>MRSRRVDVMDVMNRLILAMDLMNRDDALRVTGEVREYIDTVKIGYPLVLSEGMDIIAEFRKRFGCRIIADFKVADIPETNEKICRATFKAGADAITVHGFPGADSVRACLNVAEEMGREVFLLTEMSHPGAEMFIQGAADEIARMGVDLGVKNYVGPSTRPERLSRLREIIGQDSFLISPGVGAQGGDPGETLRFADAIIVGRSIYLADNPAAA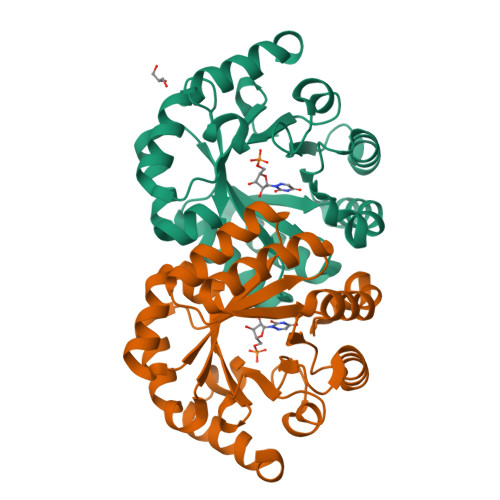AAGIIESIKDLLNP[2x]>[5x]MSEAAQTLDGWY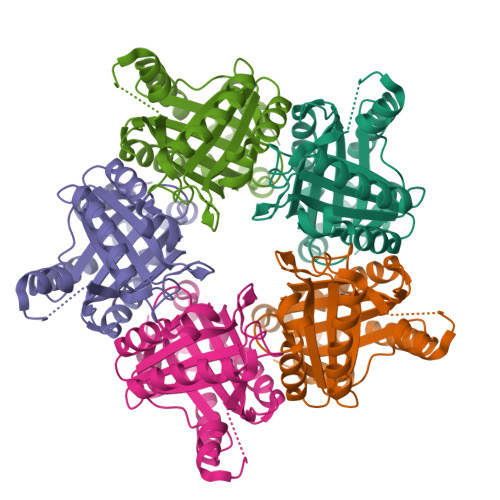CLHDFRTIDWSAWKTLPNEEREAAISEFLALVDQWETTESEKQGSHAVYTIVGQKADILFMILRPTLDELHEIETALNKTKLADYLLPAYSYVSVVELSNYLASGSEDPYQIPEVRRRLYPILPKTNYICFYPMDKRRQGNDNWYMLSMEQRRELMRAHGMTGRKYAGKVTQIITGSVGLDDFEWGVTLFSDDALQFKKLVYEMRFDEVSARFGEFGSFFVGTRLPMENVSSFFHV alpha-Diphosphopyridine nucleotide | C21 H27 N7 O14 P2 | 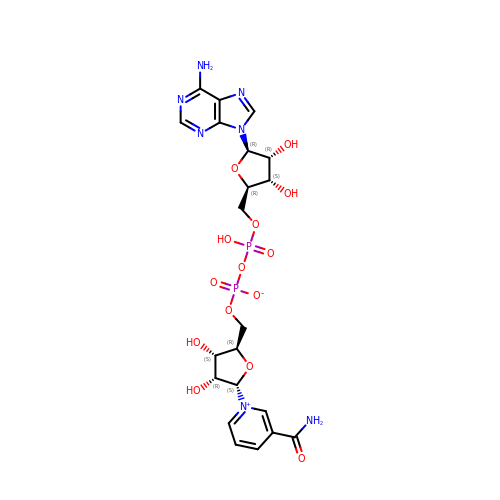BAWFJGJZGIEFAR-OPDHFMQKSA-N>[4x]MGHHHHHHGENLYFQGSAVRVQATLLPLPASETRSTVDRLKKLRLITAIKTPYL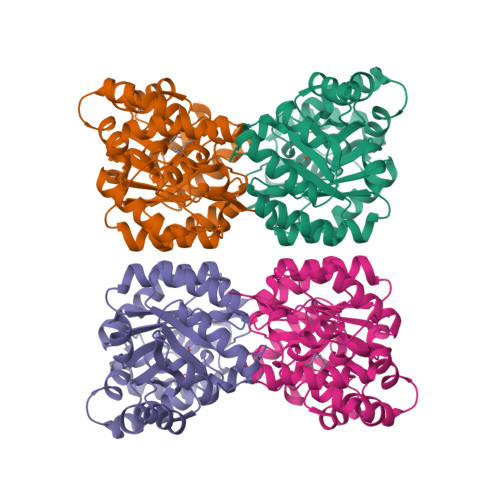ANGKFDLPAYDALVSHQIENGVEGLIVGGTTGEGHLMSWDEHVMLIAHTVNAFGDKTAVIGNTGSNSTREALHATEQGFAVGMHASLQINPYYGKTSKAGLLNHFNAVLNEGPAVVYNVPGRTGQDIPDDVVMEICQHSNFLGMKECTGNSRIKNYTSKGVNCWSGNDDESHDARHSNGAVGVISVTSNVIPGLMHKLMHGSPDPQLNADLKELMAWMFCEPNPISLNTALAMCGLARPVFRLPYVPLSRAQREKGAVLLNKVQEHIPGCKSVRVMEDHEFILVGRH> AMWTTNIIKTPRGKFEYFLKGEGPPLCVTHLYSEYNDNGNTFANPFTDHYSVYLVNLKGCGNSDSAKNDSEYSMTETIKDLEAIREALYINKWGFAGHSAGGMLALVYATEAQESLTKIIVGGAAASKEYASHKDSIYCSKNVKFNRIVSIMNALNDDSTVQEERKAL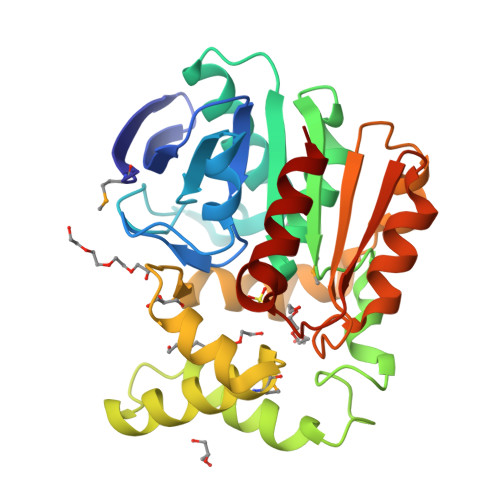SREWALMSFYSEEKLEEALKLPNSGKTVGNRLNYFRQVEYKDYDVRQKLKFVKIPSFIYCGKHDVQCPYIFSCEIANLIPNATLTKFEESNHNPFVEEIDKFNQFVNDTL>[2x]GPHMDPTAGSKKEPGGGAATEEGVNRIAVPKPPSIEEFSIVKPISRGAFGKVYLGQKGGKLYAVKVVKKADMINKNMTHQVQAERDALALSKSPFIVHL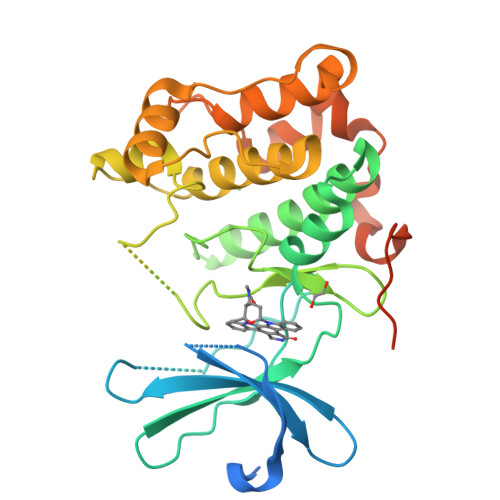YYSLQSANNVYLVMEYLIGGDVKSLLHIYGYFDEEMAVKYISEVALALDYLHRHGIIHRDLKPDNMLISNEGHIKLTDFGLSKVTLNRDINMMDILTTRTFCGTPDYLAPELLLGRAHGPAVDWWALGVCLFEFLTGIPPFNDETPQQVFQNILKRDIPWPEGEEKLSDNAQSAVEILLTIDDTKRAGMKELKRHPLFSDVDWENLQHQTMPFIPQPDDETDTSYFEARNTAQHLTVSGFSL4-({4-[3-(piperidin-1-ylcarbonyl)phenyl]pyrimidin-2-yl}amino)benzenesulfonamide | C22 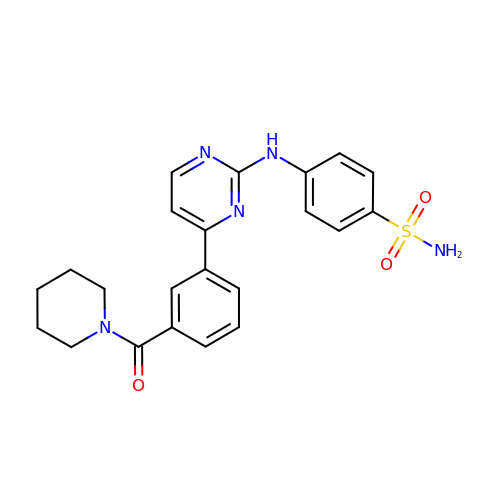H23 N5 O3 S | AMGRGTYETFMYTK-UHFFFAOYSA-N>[4x]MFKIGSVLKQIRQELNYHQIDLYSGIMSKSVYIKVEADSRPISVEELSKFSERLGVNFFEILNRAGMNTKSVNETGKEKLLISKIFTNPDLFDKNFQRIEPKRLTSLQYFSIYLGYISIAH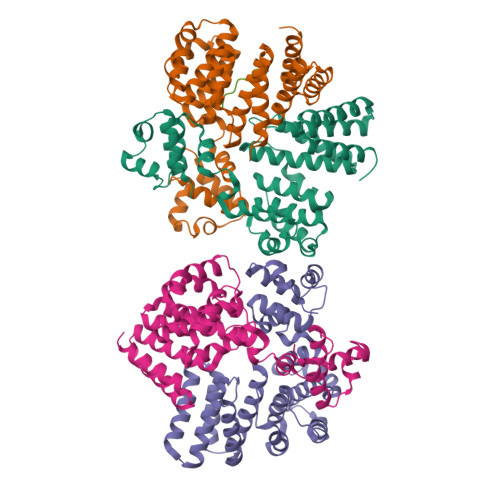HYNIEVPTFNKTITSDLKHLYDKRTTFFGIDYEIVSNLLNVLPYEEVSSIIKPMYPIVDSFGKDYDLTIQTVLKNALTISIMNRNLKEAQYYINQFEHLKTIKNISINGYYDLEINYLKQIYQFLTDKNIDSYLNAVNIINIFKIIGKEDIHRSLVEELTKISAKEKFTPPKEVTMYYENYVAIENNPIPEIKEQS;> AITLIFI> GVA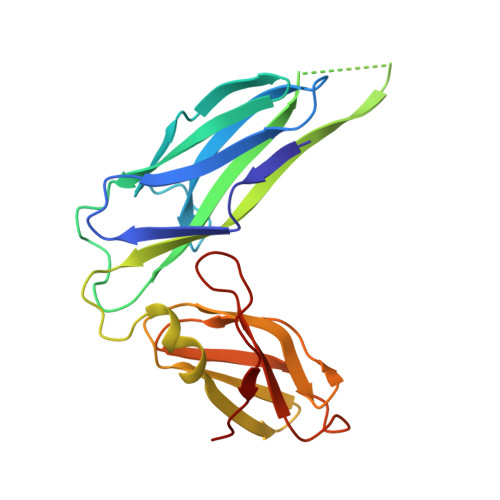LGATRVIYPAGQKQEQLAVTNNDENSTYLIQSWVENADGVKDGRFIVTPPLFAMKGKKENTLRILDATNNQLPQDRESLFWMNVKAIPSMDKSKLTENTLQLAIISRIKLYYRPAKLALPPDQAAEKLRFRRSANSLTLINPTPYYLTVTELNAGTRVLENALVPPMGESTVKLPSDAGSNITYRTINDYGALTPKMTGVME>MATYKVKDVTTGAEIEVPDDKYILDEFEKQGVNLPYSCRAGACSSCVALISSGEVDQSDGSFLSEKQEKKYILTCCSYPKSDCTIETGYEDKILEDFEIELAETGLEFFNDLKDSLPRSGEILSGVTAPFEAFDHYLFGNGVERSININDVGFNINVSQIPPIMSLLNGKNVGRFDIGSDFVRNTALDGYSVAAYLGNITMRTEGVLNVKSDGTWQYEGVIRSYNDTYDANPSTHRGALGEWATGVLNNLSGTPYEIRIPGELKIKENGKKLEHHHHHH[2x]

Pectocin M1 and M2 consist of an M-class cytotoxic domain with lipid II degrading activity, fused to a plant-like ferredoxin domain (Grinter et al., 2012a; 2013,). This ferredoxin domain, which contains an intact [2Fe-2S] iron–sulphur cluster, substitutes for the helical receptor binding domain and IUTD of the M-class bacteriocins discussed above, that are required to deliver the cytotoxic domain to the periplasm. We have previously demonstrated that Pectobacterium spp. are able to acquire iron directly from plant ferredoxin under iron-limiting conditions through a receptor mediated process and that the bacteriocins pectocin M1 and M2 parasitize this system for cell entry through presentation of a ferredoxin domain (Grinter et al., 2013). The lack of an IUTD indicates that the ferredoxin-containing pectocins utilize an existing ferredoxin uptake mechanism to cross the OM, without direct interaction with the Tol or Ton complexes in the periplasm.

The bimodal distribution of the selected ensembles suggests discrete populations in solution, the more compact of which is similar to the conformation observed in the P21 crystals of pectocin M2. In an attempt to capture the more elongated conformation in crystallo, thus validating our solution scattering and modelling data, we repeated crystallization of pectocin M2. A form with the radically different space group of P3121 was chosen for optimization, which yielded crystals diffracting to 1.86 Å. As an alternative domain arrangement to the P21 form was expected, data from this crystal form were again phased using anomalous data from the metal centres of the [2Fe-2S] cluster. During model building from these data it was immediately apparent that in this crystal form pectocin M2 did indeed adopt an elongated conformation. The calculated Rg and Dmax for this structure were 28 and 97 Å respectively. These values correlate well with the extended population from the DMD simulation, suggesting that this structure is representative of the second elongated pool indentified by our modelling. Alignment of this elongated (P3121) form and the original P21 form, based on their cytotoxic or ferredoxin domains, show a major difference in the relative orientations of these domains. As the elongated conformation of pectocin M2 has comparable dimensions along its length we manually docked this model into the barrel domain of the hemophore receptor HasR, a TonB-dependent receptor shown to be responsible for importation of the relatively bulky substrate, haem. This docking illustrates that pectocin M2 in its elongated conformation could traverse the lumen of such a receptor to gain entry to the cell, with the flexibility of pectocin M2 observed in solution allowing the protein to adapt to the shape of the lumen of its transporter during importation.>[2x]GAMGSKFSVEEYLVHALQGSVSSGQAHSLTSLAKTWAARGSRSREPSPKTEDNEGVLLTEKLKPVDYEYREEVHWATHQLRLGRGSFGEVHRMEDKQTGFQCAVKKVRLEVFRAEELMACAGLTSPRIVPLYGAVREGPWVNIFME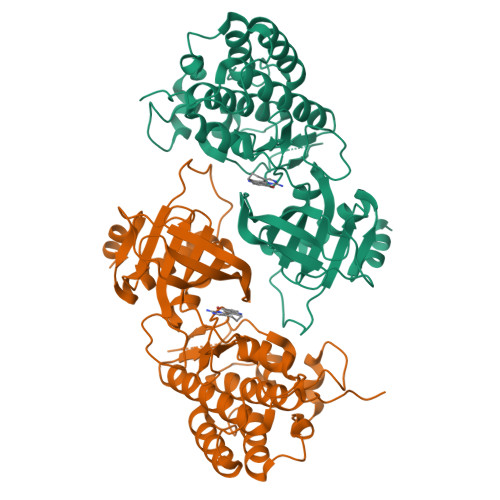LLEGGSLGQLVKEQGCLPEDRALYYLGQALEGLEYLHSRRILHGDVKADNVLLSSDGSHAALCDFGHAVCLQPDGLGKDLLTGDYIPGTETHMAPEVVLGRSCDAKVDVWSSCCMMLHMLNGCHPWTQFFRGPLCLKIASEPPPVREIPPSCAPLTAQAIQEGLRKEPIHRVSAAELGGKVNRALQQVGGLKSPWRGEYKEPRHPPPNQA> MRPERLTVRNFLGLKNVDIEFQSGITVVEGPNGAGKSSLFEAISFALFGNGIRYPNSYDYVNRNAVDGTARLVFQFERGGKRYEIIREINALQRKHNAKLSEILENGKKAAIAAKPTSVKQEVEKILGIEHRTFIRTVFLPQGEIDKLLISPPSEITEIISDVFQSKETLEKLEKLLKEKMKKLENEISSGGAGGAGGSLEKKLKEMSDEYNNLDLLRKYLFDKSNFSRYFTGRVLEAVLKRTKAYLDILTNGRFDIDFDDEKGGFIIKDWGIERPARGLSGGERALISISLAMSLAEVASGRLDAFFIDEGFSSLDTENKEKIASVLKELERLNKVIVFITHDREF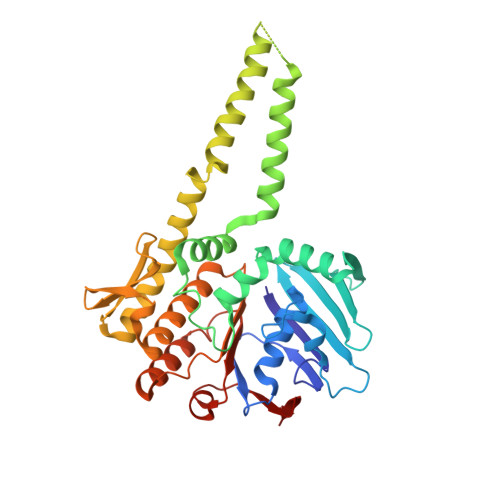SEAFDRKLRITGGVVVNE> ASA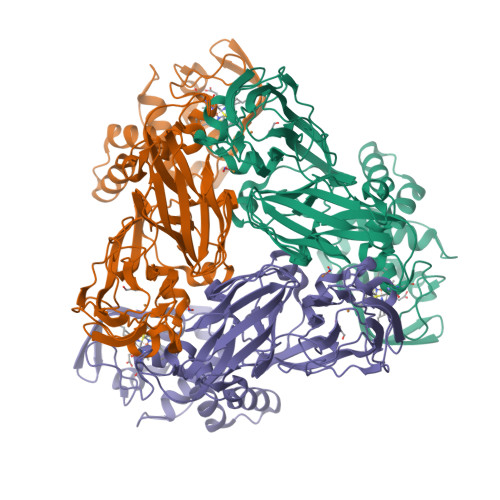KLPGDFGPPRGEPIHAVLTSPPLVPPPVNRTYPAKVIVELEVVEKEMQISEGVSYTFWTFGGTVPGSFIRVRQGDTVEFHLKNHPSSKMPHNIDLHGVTGPGGGAASSFTAPGHESQFTFKALNEGIYVYHCATAPVGMHIANGMYGLILVEPPEGLPKVDHEYYVMQGDFYTAGKYREKGLQPFDMEKAIDERPSYVLFNGAEGALTGDKALHAKVGETVRIFVGNGGPNLVSSFHVIGAIFDQVRYEGGTNVQKNVQTTLIPAGGAAVVKFTARVPGSYVLVDHSIFRAFNKGAMAILKIDGAENKLVYSGKELDSVELGDRAAPNMSAVTKATQASVSGTLTVQDQVQAGRALFAGTCSVCHQGNGAGLPGVFPPLAKSDFLAADPKRAMNIVLHGLNGKIKVNGQEYDSVMPPMTQLNDDEVANILTYVLNSWDNPGGRVSAEDVKKVRAQPAPAKAVAEH> MGSSHHHHHHSSENLYFQGHMNEIYQKAKHIKLFAMDVDGILSDGQIIYNSEGTETKAFYVQDGLGLQALKQSGIILAIITGRSSAMVDRRAKELGI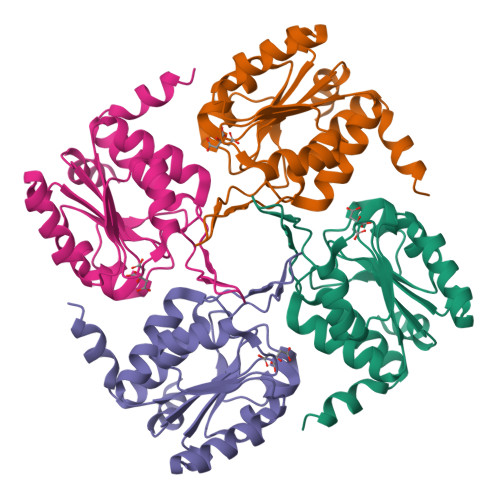SHIIQGQDDKLTALVGLTKKLGIELSHCAYIGDDLPDLKAVREAGFGISVPNGCEQTRAVSDYITTKTGGNGAVREVCELILKAQNNFDAFIATFQ> MAFVVTDNCIKCKYTDCVEVCPVDCFY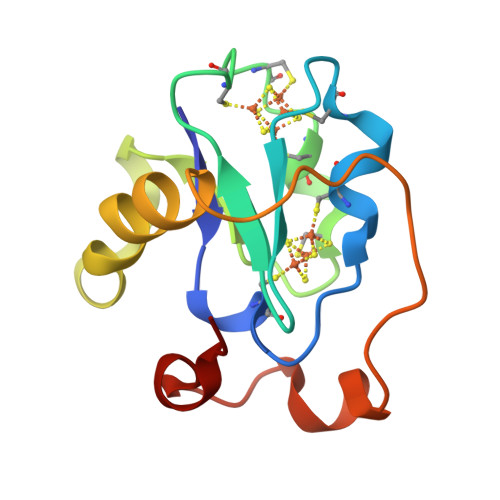EGPNFLVIHPDECIDCALCEPECAAQAIFSEDEVPEDMQEFIQLNAELAEVWPNITEKKDPLPDAEDWDGVKGKLQHLER>[3x]METKMTSFYKITAYNSQALYFWGTDADVDRYVDWLNRDREINVYAAEAIPEAEWAQYEGRDDVLSGEECGWDDFMSAEA

Anti-CRISPR proteins (Acrs) are naturally occurring inhibitors of CRISPR–Cas systems that have been identified in various bacterial and archaeal species. AcrIC9 is the most recently identified member of the AcrIC family that inhibits the type IC CRISPR–Cas system. Analysis and comparison of its structure with structural homologs indicate that AcrIC9 belongs to DNA-mimic Acrs that directly bind to the cascade complex and hinder the target DNA from binding to the cascade.

AcrIC9 was successfully crystalized as a single crystal diffracting at 2.4 Å under synchrotron radiation. The crystal belongs to space group P3112, with three molecules present in the asymmetric unit (ASU). The final structural models contain residues Met5 to Ser76 for molecule A and Met5 to Glu78 for molecules B and C [Fig. 2(a)]. Since the electrostatic surface features of a protein are sometimes correlated with its function, we analyzed them to obtain information about the working mechanism of AcrIC9. The results of this analysis indicate that the surface of AcrIC9 is highly acidic [Fig. 2(d)]. Therefore, this highly acidic surface feature may indicate that AcrIC9 is one of the DNA-mimic Acrs. Moreover, the long α2–α3 connecting loop and C-terminal loop exhibit a relatively high B-factor value (average of 54.3 Å2) compared with the low B factor (average of 40.2 Å2) of the overall structure. This indicates that although a major part of AcrIC9 is rigid in solution, it contains a relatively flexible α2–α3 connecting loop [Fig. 2(f)]. We performed SPR spectroscopy to confirm the interaction between AcrIC9 and the cascade. As shown in Fig. 4(c) and Table S1 of the supporting information, AcrIC9 binds to the cascade complex with a KD value of 4.32 nM.Human mitochondrial nuclease EXOG (hEXOG) is important for mtDNA integrity. hEXOG depletion selectively increases lesions in mtDNA, but has no effect on chromosomal DNA. Human EXOG shares sequence homology with members of ββα-Me nuclease family, which contains nonspecific endonucleases. The catalytic Core domain of hEXOG is identical to EndoG, but its C-terminal extension forms a unique Wing domain that converts the enzyme from a nonspecific endonuclease into a DNA-geometry-specific exonuclease. Conversely, in mitochondrial LP-BER, the nuclease reaction occurs before DNA synthesis: hEXOG processes the 5′-end of DNA downstream of the lesion, generating an optimal substrate for DNA synthesis catalysed by Pol γ.

Apo hEXOG is a symmetrical homodimer. Each monomer contains a Core domain that is extremely similar to that of EndoG (r.m.s.d.=0.8 Å), and a helical-bundle Wing domain that corresponds to the C-terminal extension. The N terminus of each hEXOG monomer undergoes a domain-swap where the folding of the region is identical to that in EndoG, but the involved residues are from the opposing monomer rather than from the same monomer in EndoG: the residues 58KAVLEQFGFPLT70 (hydrophobic residues are bold) of one monomer collapse on a hydrophobic patch (277GLVFFPHL284) of the opposing monomer 30 Å away. The swapped domains represent 45% of the total dimer interface in hEXOG, and thus contribute substantially to dimer stability. A Mg2+ is found in each active site, forming octahedron coordination with five water molecules and Nδ of N171. In contrast to the completely solvent exposed active site of EndoG, the active site of hEXOG is an enclosed V-shaped cleft. The cleft, measuring 32–35 Å in depth and 15 Å in width, is lined with positively charged residues from both Core and Wing domains, and is both electrostatically and dimensionally capable of accommodating dsDNA at its end. Interestingly, R138 and R314 bind two sulfate molecules in the apo structure in an essentially identical manner to the phosphdiester backbone of substrate DNA, reflecting their affinity for negative charges.

>[2x]MKAVLEQFGFPLTGTEARCYTNHALSYDQAKRVPRWVLEHISKSKIMGDADRKHCKFKPDPNIPPTFSAFNEDYVGSGWSRGHMAPAGNNKFSSKAMAETFYLSNIVPQDFDNNSGYWNRIEMYCRELTERFEDVWVVSGPLTLPQTRGDGKKIVSYQVIGEDNVAVPSHLYKVILARRSSVSTEPLALGAFVVPNEAIGFQPQLTEFQVSLQDLEKLSGLVFFPHLDRTSDIRNICSVDTCKLLDFQEFTLYLSTRKIEGARSVLRLEKIMENLKNAEIEPDDYFMSRYEKKLEELKAKEQSGTQIRKPSHHHHHH> MAVTDLSLTNSSLMPTLNPMIQQLALAIAASWQSLPLKPYQLPEDLGYVEGRLEGEKLVIENRCYQTPQFRKMHLELAKVGKGLDILHCVMFPEPLYGLPLFGCNIVAGPGGVSAAIADLSPTQSDRQLPAAYQKSLAELGQPEFEQQRELPPWGEIFSEYCLFIRPSNVTEEERFVQRVVDFLQIHCHQSIVAEPLSEAQTLEHRQGQIHYCQQQQKNDKTRRVLEKAFGEAWAERYMSQVLFDVIQ

PcyA, a ferredoxin-dependent bilin pigment reductase, catalyzes the site-specific reduction of the two vinyl groups of biliverdin (BV), producing phycocyanobilin. PcyA catalyzes a two-step reduction reaction: in the first step, the D-ring vinyl group of BV is reduced using two electrons and two protons to produce the reaction intermediate, 181, 182-dihydrobiliverdin (18EtBV), and in the second step, the A-ring of 18EtBV is reduced using two electrons and two protons to synthesize PCB. In the case of PcyA, three residues, namely, glutamate, histidine, and aspartate (Glu76, His88, and Asp105 in Synechocystis PcyA), present near the D- and A-rings of BV, are essential for the PcyA reaction. Here, we performed neutron crystallography and quantum chemical analysis of the D105N–BV and I86D–BV complexes to determine the protonation states of BV and the surrounding residues and study the correlation between the absorption spectra and protonation states around BV.

The D105N mutant, in which aspartate at position 105 is substituted with asparagine, was reported to be only approximately 10% as active as wildtype (WT) PcyA. Spectroscopic analysis also revealed that D105N receives an electron to produce BV radicals. However, because of the mutation, enzymatic catalysis does not proceed, as the proton transfer from the carboxy side chain of Asp105 to the substrate is no longer possible. In the previously determined absorption spectra of the PcyA D105N and I86D mutants, complexed with BV, a peak at 730 nm, observed in the WT, disappeared and increased, respectively. Neutron structures elucidated that BV in the D105N mutant is in a neutral state, whereas that in the I86D mutant is dominantly in a protonated state. Our quantum mechanics/molecular mechanics calculations of the absorption spectra showed that the spectral change in D105N arises from Glu76 deprotonation, consistent with the neutron structure. Glu76 and His88 showed different hydrogen bonding with surrounding residues compared with WT PcyA, further explaining why D105N and I86D have much lower activities for phycocyanobilin synthesis than the WT PcyA. The neutron structures of PcyA D105N–BV and I86D–BV at room temperature were refined to 2.10 Å and 2.00 Å resolutions, respectively. The R-factor and free R-factor for the D105N–BV structures were 16.51% and 18.00%, respectively, while those for the I86D–BV structures were 17.25% and 20.82%, respectively.> SNAMKTYKVAVLAGDGIGPLVMKEALKILTFIAQKYNFSFELNEAKIGGASIDAYGVALSDETLKLCEQSDAILFGSVGGPKWDNLPIDQRPERASLLPLRKHFNLFANLRPCKIYESLTHASPLKNEIIQKGVDILCVRELTGGIYFGKQDLGKESAYDTEIYTKKEIERIARIAFESARIRKKKVHLIDKANVLASSILWREVVANVAKDYQDINLEYMYVDNAAMQIVKNPSIFDVMLCSNLFGDILSDELAAINGSLGLLSSASLNDKGFGLYEPAGGSAPDI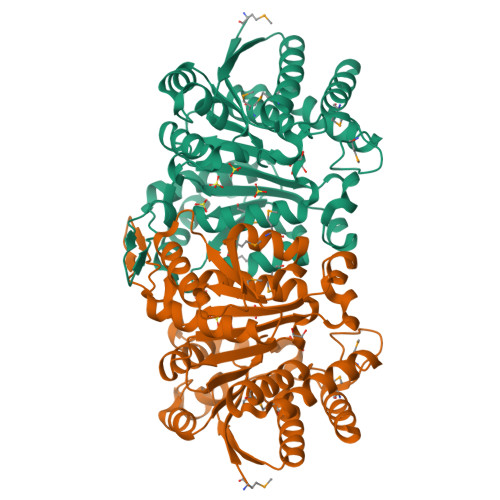AHLNIANPIAQILSAALMLKYSFKEEQAAQDIENAISLALAQGKMTKDLNAKSYLNTDEMGDCILEILKENDNG>HHHHHHMKTRIHVVQGDITKLAVDVIVNAANPSLMGGGGVDGAIHRAAGPALLDACL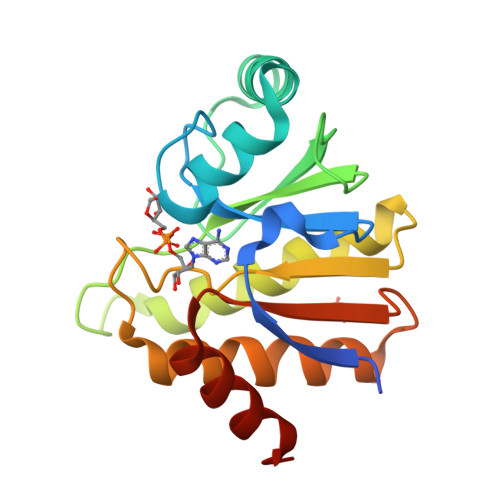KVRQQQGDCPTGHAVITLAGDLPAKAVVHTVGPVWRGGEQNEDQLLQDAYLNSLRLVAANSYTSVAFPAISTGVAGYPRAAAAEIAVKTVSEFITRHALPEQVYFVCYDEENAHLYERLLTQQGDE[18x]(2S)-azetidine-2-carboxylic 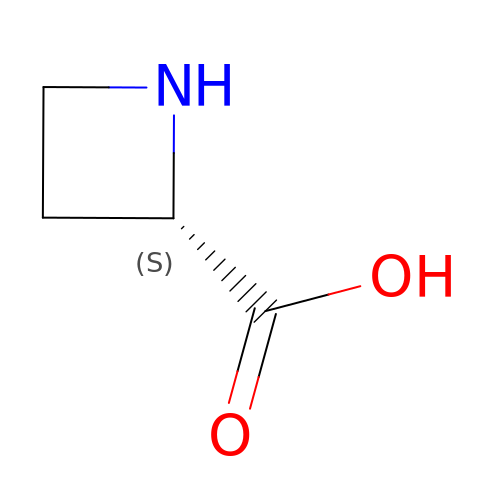acid | C4 H7 N O2 | IADUEWIQBXOCDZ-VKHMYHEASA-N>MAEILRAENIKKVIRGYEILKGISLSVKKGEFVSIIGASGSGKSTLLYILGLLDAPTEGKVFLEGKEVDYTNEKELSLLRNRKLGFVFQFHYLIPELTALENVIVPMLKMGKPKKEAKERGEYLLSELGLGDKLSRKPYELSGGEQQRVAIARALANEPILLFADEPTGNLDSANTKRVMDIFLKINEGGT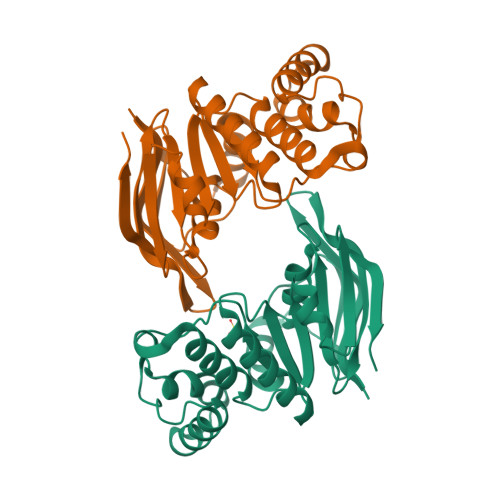SIVMVTHERELAELTHRTLEMKDGKVVGEITRV[2x]>[2x]VKTQRVVITPGEPAGIGPDLVVQLAQREWPVELVVCADATLL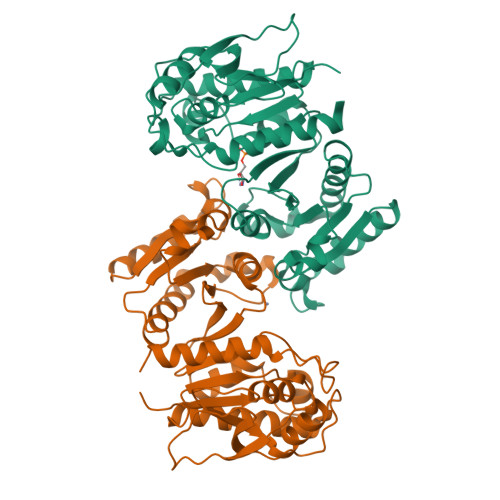TNRAAMLGLPLTLRPYSPNSPAQPQTAGTLTLLPVALRAPVTAGQLAVENGHYVVETLARACDGCLNGEFAALITGPVHKGVINDAGIPFTGHTEFFEERSQAKKVVMMLATEELRVALATTHLPLRDIADAITPALLHEVIAILHHDLRTKFGIAEPRILVCGLNPHAGEGGHMGTEEIDTIIPVLNELRAQGMKLNGPLPADTLFQPKYLDNADAVLAMYHDQGLPVLKYQGFGRGVNITLGLPFIRTSVDHGTALELAGRGKADVGSFITALNLAIKMIVNTQ>MDDRLFRNAMGKFATGVTVITTELNGAVHGMTANAFMSVSLNPKLVLVSIGEKAKMLEKIQQSKKYAVNILSQDQKVLSMNFAGQLEKPVDVQFEELGGLPVIKDALAQISCQVVNEVQAGDHTLFIGEVTDI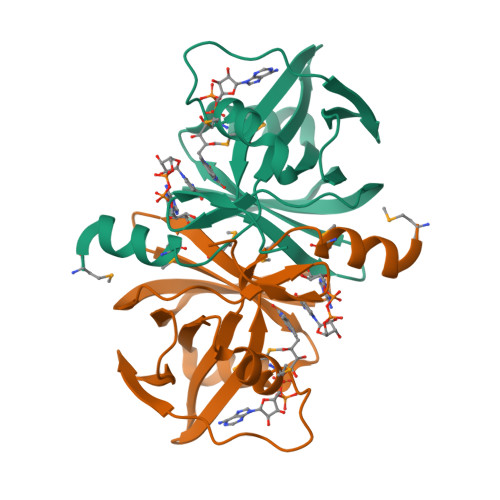KITEQDPLLFFSGKYHQLAQNEKVETSS[8x]>SPEFMVKAKSWTLKKHFQGKPTQSDFELKTVELPPLKNGEVLLEALFLSVDPYMRIASKRLKEGAVMMGQQVARVVESKNSAFPAGSIVL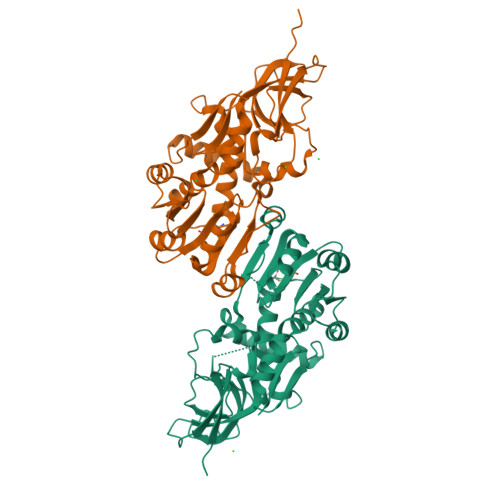AQSGWTTHFISDGKGLEKLLTEWPDKLPLSLALGTIGMPGLTAYFGLLEVCGVKGGETVLVSAAAGAVGSVVGQIAKLKGCKVVGAAGSDEKIAYLKQIGFDAAFNYKTVNSLEEALKKASPDGYDCYFDNVGGEFLNTVLSQMKDFGKIAICGAISVYNRMDQLPPGPSPESIIYKQLRIEGFIVYRWQGDVREKALRDLMKWVLEGKIQYHEHVTKGFENMPAAFIEMLNGANLGKAVVTA[2x]>SNAMQRYLWQQADGKRHVYDTARHRVQAGRPFTALCGETVTPQTERGDLTAGLWFDGECPVCTIALAKALGWPVREISDLAHRFDWSPALITRLAEVLHCSFG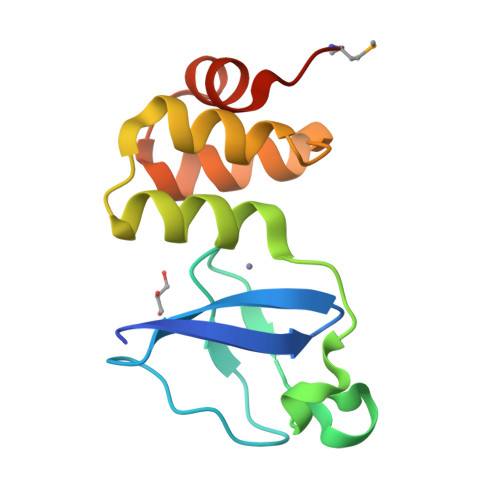EVVELTGARMVDA[3x]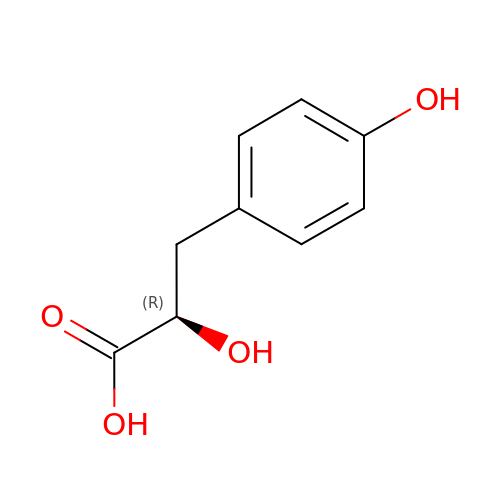(2R)-2-HYDROXY-3-(4-HYDROXYPHENYL)PROPANOIC ACID | C9 H10 O4 | JVGVDSSUAVXRDY-MRVPVSSYSA-N heptyl 2-fluoro-alpha-D-mannopyranoside | C13 H25 F O5 | 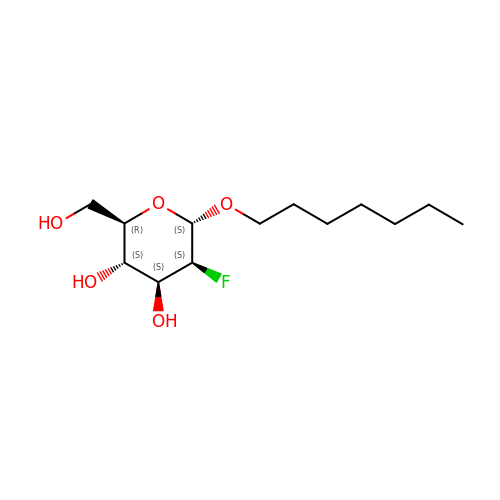UNCNEFLGGSGWLT-MLGHIDQZSA-N> MSIQHFRVALIPFFAAFCLPVFAHPETLVKVKDAEDQLGARVGYIELDLNSGKILESFRPEERFPMMXTFKVLLCGAVLSRIDAGQEQLGRRIHYSQNDLVEYSPVTEKHLTDGMTVRELCSAAITMSDNTAANLLLTTIGGPKELTAFLHNMGDHVTRLDRWNPELNEAI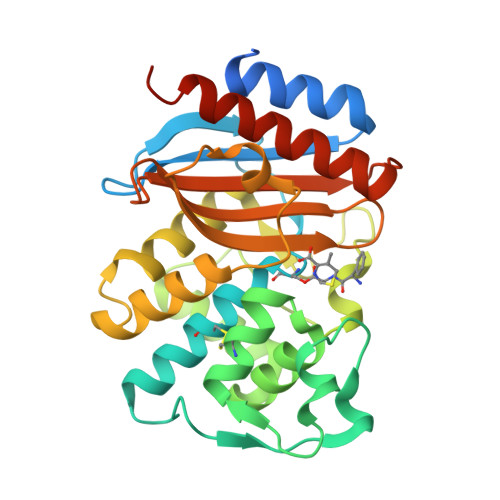PNDERDTTMPVAMATTLRKLLTGELLTLASRQQLIDWMEADKVAGPLLRSALPAGWFIADKSGAGERGSRGIIAALGPDGKPSRIVVIYTTGSQATMDERNRQIAEIGASLIKHWAAALEHHHHHH>[6x]MAHHHHHHMSTLTNSLKQRLRDGDEPLYGLWLSLGSDSAAEALAHAGYDWLCIDMEHAPNDSRDVASQLRAIAAAHLPSEPVVRVPAREPWLVKRALDAGARTLMFPCIETPDDAAHAVRLTRFPSPESPDGLRGVAGMVRAAAFGMRRDYLQTANAQVAVIVQVESARGVDEVERIAATPGVDCLFVGPADLAASLGHLGDIRHPDVETAMARVLAAGKQAGVAVGIFAGDTAAARQYREAGYRL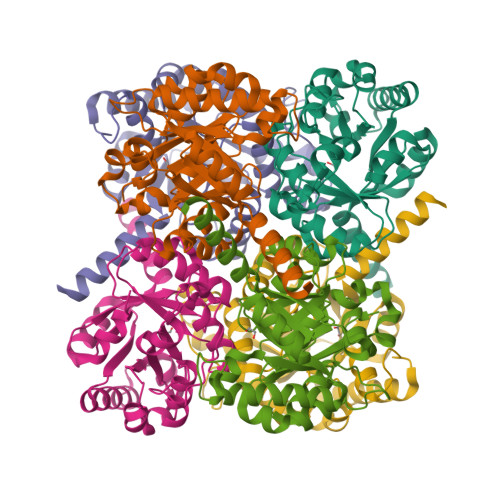ITVSADVSWLLRATRQALQEVRS>MAGAIENARKEIKRISLEDHAESEYGAIYSVSGPVVIAENMIGCAMYELVKVGHDNLVGEVIRIDGDKATIQVYEETAGLTVGDPVLRTGKPLSVELGPGLMETIYDGIQRPLKAIKEESQSIYIPRGIDTPALDRTIKWQFTPGKFQVGDHISGGDIYGSVFENSLISSHKILLPPRSRGTITWIAPAGEYTLDEKILEVEFDGKKSDFTLYHTWPVRVPRPVTEKLSADYPLLTGQRVLDALFPCVQGGTTCIPGAFGCGKTVISQSLSKYSNSDAIIYVGCGERGNEMAEVLMEFPELYTEMSGTKEPIMKRTTLVANTSNMPVAAREASIYTGITLAEYFRDQGKNVSMIADSSSRWAEALREISGRLGEMPADQGFPAYLGAKLASFYERAGKAVALGSPDRTGSVSIVAAVSPAGGDFSDPVTTATLGITQVFWGLDKKLAQRKHFPSINTSVSYSKYTNVLNKFYDSNYPEFPVLRDRMKEILSNAEELEQVVQLVGKSALSDSDKITLDVATLIKEDFLQQNGYSTYDAFCPIWKTFDMMRAFISYHDEAQKAVANGANWSKLADSTGDVKHAVSSSKFFEPSRGEKEVHGEFEKLLSTMQERFAESTDDYKDHDGDYKDHDIDYKDDDDK[3x];>[3x]MVLSDKELFAINKKAVEQGFNVKPRLNYNTVSGVNGPLVILEKVKFPRYNEIVNLTLPDGTVRQGQVLEIRGDRAIVQVFEGTSGIDVKKTTVEFTGESLRIPVSEDMLGRIFDGSGRPIDNGPKVFAEDYLDINGSPINPYARIYPEEMISTGVSAIDTMNSIARGQKIPIFSASGLPHNEIAAQICRQAGLVRPTKDVHDGHEENFSIVFAAMGVNLETARFFKQDFEENGSLERTSLFLNLANDPTIERIITPRLALTTAEYLAYQTERHVLTILTDMSSYADALREVSAAREEVPGRRGYPGYMYTDLSTIYERAGRVEGRNGSITQIPILTMPNDDITHPIPDLTGYITEGQIFVDRQLHNKGIYPPINVLPSLSRLMKSAIGEGMTRKDHGDVSNQLYAKYAIGKDAAAMKAVVGEEALSIEDKLSLEFLEKFEKTFITQGAYEDRTVFESLDQAWSLLRIYPKEMLNRISPKILDEFYDRARDDADEDEEDPDTRSSGKKKDASQEESLI;>MSSAITALTPNQVNDELNKMQAFIRKEAEEKAKEIQLKADQEYEIEKTNIVRNETNNIDGNFKSKLKKAMLSQQITKSTIANKMRLKVLSAREQSLDGIFEETKEKLSGIANNRDEYKPILQSLIVEALLKLLEPKAIVKALERDVDLIESMKDDIMREYGEKA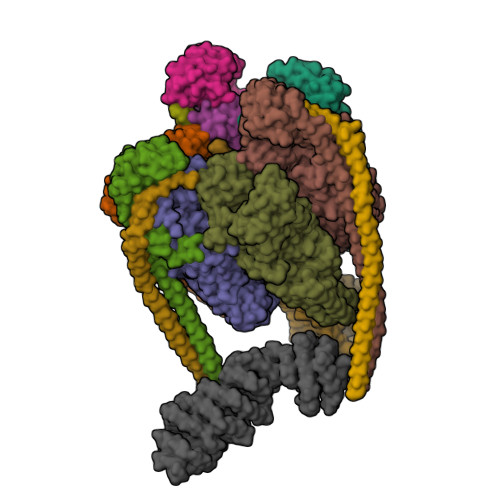QRAPLEEIVISNDYLNKDLVSGGVVVSNASDKIEINNTLEERLKLLSEEALPAIRLELYGPSKTRKFFD[3x];>[3x]MSQKNGIATLLQAEKEAHEIVSKARKYRQDKLKQAKTDAAKEIDSYKIQKDKELKEFEQKNAGGVGELEKKAEAGVQGELAEIKKIAEKKKDDVVKILIETVIKPSAEVHINAL;> MSGNREQVFPTRMTLGLMKTKLKGANQGYSLLKRKSEALTKRFRDITKRIDDAKQKMGRVMQTAAFSLAEVSYATGENIGYQVQESVSTARFKVRARQENVSGVYLSQFESYIDPEINDFRLTGLGRGGQQVQRAKEIYSRAVETLVELASLQTAFIILDEVIKVTNRRVNAIEHVIIPRTENTIAYINSELDELDREEFYRLKKVQEKKQNETAKLDAEMKLKRDRAEQDASEVAADEEPQGETLVADQEDDVIF;> MAEKRTLIAVIADEDTTTGLLLAGIGQITPETQEKNFFVYQEGKTTKEEITDKFNHFTEERDDIAILLINQHIAENIRARVDSFTNAFPAILEIPSKDHPYDPEKDSVLKRVRKLFGE;> MGATKILMDSTHFNEIRSIIRSRSVAWDALARSEELSEIDASTAKALESILVKKNIGDGLSSSNNAHSGFKVNGKTLIPLIHLLSTSDNEDCKKSVQNLIAELLSSDKYGDDTVKFFQEDPKQLEQLFDVSLKGDFQTVLISGFNVVSLLVQNGLHNVKLVEKLLKNNNLINILQNIEQMDTCYVCIRLLQELAVIPEYRDVIWLHEKKFMPTLFKILQRATDSQLATRIVATNSNHLGIQLQYHSLLLIWLLTFNPVFANELVQKYLSDFLDLLKLVKITIKEKVSRLCISIILQCCSTRVKQHKKVIKQLLLLGNALPTVQSLSERKYSDEELRQDISNLKEILENEYQELTSFDEYVAELDSKLLCWSPPHVDNGFWSDNIDEFKKDNYKIFRQLIELLQAKVRNGDVNAKQEKIIIQVALNDITHVVELLPESIDVLDKTGGKADIMELLNHSDSRVKYEALKATQAIIGYTFK Human SIDT1 and SIDT2 are closely related members of the SID-1 transmembrane family, and have been implicated in various biological processes such as glucose and lipid metabolism, innate immunity, and tumorigenesis. Here, we present the cryo-electron microscopy (cryo-EM) structures of human SIDT1 and SIDT2. Both structures reveal an overall architecture of a dimeric arrangement composed of an extracellular domain (ECD) rich in β-strands and a transmembrane domain (TMD) with 11 passes, highlighting the remarkable structural congruence. Importantly, the ECDs of SIDT1 and SIDT2 bind synthetic plant-derived miRNA only under acidic conditions.

The SIDT1 ECD consists of two subdomains, ECD1 and ECD2, connected by a flexible loop. A disulfide bond between C130 of ECD1 and C222 of ECD2, along with another pair of disulfide bonds between C212 and C271 on ECD2, contributes to the stability of SIDT1. Bioinformatics analysis predicted eight N-glycosylation sites in SIDT1, with three glycosylation sites resolved in the EM map. The dimer interface of the SIDT1 ECD can be divided into two regions. The first region involves hydrophobic interactions between ECD1 subdomains of two protomers, supported by hydrogen bond interactions. A conserved hydrogen bond between S105 residues is observed in SIDT1, corresponding to S92 in SIDT2. The second region involves a long loop on ECD2, connecting two β-strand sheets, with a potential hydrogen bond between H229 and N230. In addition, Q113 in SIDT1 may maintain a hydrogen bond interaction with N219 from the other protomer instead of the ionic bond interaction observed between R100 and D204 in SIDT2. In the SIDT2 ECD model, the dimerization interaction involves a buried surface area of ~1700 Å2 from each protomer, in contrast to ~1300 Å2 in the SIDT1 model, indicating differences in the proximity of the formed homodimers between SIDT1 and SIDT2, probably due to sequence variations. Sedimentation velocity analytical ultracentrifugation (SV-AUC) analysis further confirmed that SIDT1ECD exists as a monomer, with a sedimentation coefficient of 2.8 S and a molecular weight of ~44.6 kDa, while SIDT2ECD forms a dimer with a sedimentation coefficient of 4.8 S and a molecular weight of ~74.2 kDa.

>[2x]DFDHVYSGVVNLSTENIYSFNYTSQPDQVTAVRVYVNSSSENLNYPVLVVVRQQKEVLSWQVPLLFQGLYQRSYNYQEVSRTLCPSEATNETGPLQQLIFVDVASMAPLGAQYKLLVTKLKHFQLRTNVAFHFTASPSQPQYFLYKFPKDVDSVIIKVVSEMAYPCSVVSVQNIMCPVYDLDHNVEFNGVYQSMTKKAAITLQKKDFPGEQFFVVFVIKPEDYACGGSFFIQEKENQTWNLQRKKNLEVTIVPS> ELDDEDFRCVCNFSEPQPDWSEAFQCVSAVEVEIHAGGLNLEPFLKRVDADADPRQYADTVKALRVRRLTVGAAQVPAQLLVGALRVLAYSRLKELTLEDLKITGTMPPLPLEATGLALSSLRLRNVSWATGRSWLAELQQWLKPGLKVLSIAQAHSPAFSCEQVRAFPALTSLDLSDNPGLGERGLMAALCPHKFPAIQNLALRNTGMETPTGVCAALAAAGVQPHSLDLSHNSLRA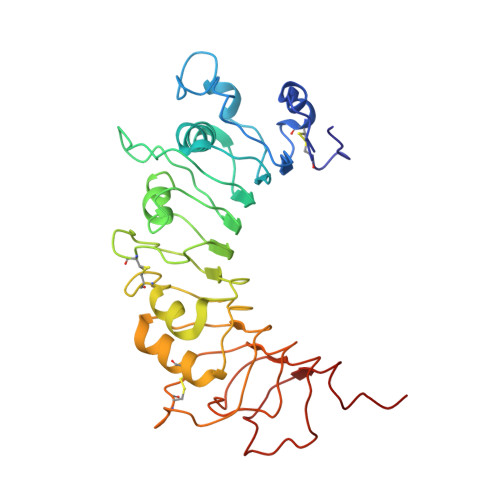TVNPSAPRCMWSSALNSLNLSFAGLEQVPKGLPAKLRVLDLSSNRLNRAPQPDELPEVDNLTLDGNPFLVPG[6-(3,4-dihydroxyphenyl)pyridin-2-yl](4-fluoro-3-hydroxyphenyl)methanone | C18 H12 F N O4 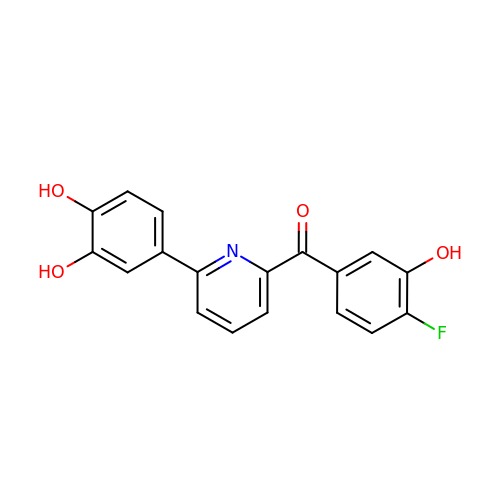| USZFAGSFWNNZLX-UHFFFAOYSA-N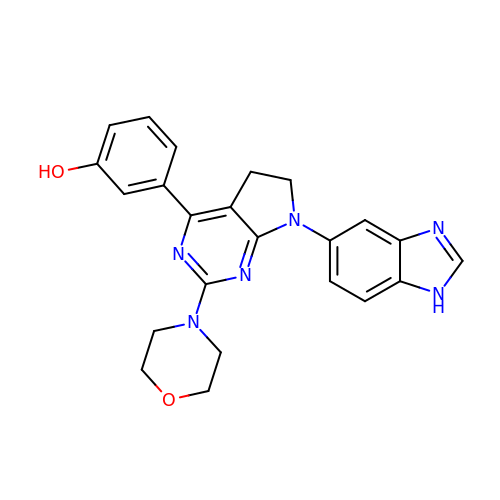3-[7-(1H-benzimidazol-5-yl)-2-(morpholin-4-yl)-6,7-dihydro-5H-pyrrolo[2,3-d]pyrimidin-4-yl]phenol | C23 H22 N6 O2 | NBBUAPYZXMAOGM-UHFFFAOYSA-N The second type of rubber oxygenase has been named latex clearing protein (Lcp). Controversial reports were published on the cofactor of Lcp from Streptomyces sp. K30 (LcpK30) and G. polyisoprenivorans VH2 (LcpVH2)23, 24 but recently iron was detected in an almost 1:1 stoichiometry in pure preparations of LcpK30 and of LcpRr, and both Lcps were identified as b-type cytochromes. The typical, α-helical tertiary structure identifies LcpK30 as a member of the globin family. However, LcpK30 contains additional subdomains at the N- and C-termini beyond the globin core that form two caps located on opposite sides of the protein.

Here we report the three-dimensional structure of LcpK30 in a closed and in an open confirmation. His198 (F13) acts as the proximal axial ligand in LcpK30 and corresponds to His (F8) of GCSGsu according to the haemoglobin nomenclature. Interestingly, distal haem ligation in LcpK30 is not provided by a histidine as in most other globins and many cytochromes, but by a lysine residue (Lys167, E7) that corresponds to (His) E11 in GCSGsu and (His) E7 in haemoglobin. The presence of two axial ligands (His198, Lys167) to the haem iron in LcpK30 prevents the direct binding of dioxygen that is required for the dioxygenase activity of the enzyme and identifies this structure as a closed and inactive form. As a consequence, a conformational change in the vicinity of the haem group is required to allow for access and binding of O2 and of the polyisoprene chain to the haem site. The transition to the closed state only bars one entrance to this tunnel, but concomitantly blocks access to the haem iron by reinstating Lys167 as a direct ligand to the metal, thus efficiently preventing the reaction of the enzyme with dioxygen. Although LcpK30 is an extracellular enzyme, this conformational switch may well represent a protective mechanism to avoid the generation of reactive oxygen species from the reduced haem cofactor in the absence of substrate molecules. In summary, the findings for LcpK30 muteins with single amino acid exchanges of residues in the active site region were in agreement with the 5-fold-coordinated (open) state of the Lys167Ala mutein and with the 6-fold coordinated (closed) state in the wild type and in the Lys167His mutein with His167 as a second axial haem ligand. These data confirm that the unusual Lys167 haem ligand stabilises the protein in the absence of substrate in the closed state. z = 3.06 is typical for a low spin haem (Fe3+, S = 1/2), presumably from the closed state of the enzyme with Lys167 completing the octahedral coordination of the metal ion.

>[2x]PLWTWSPSASVAGTGVGVDPEYVWDEEADPVLAAVIDRGEVPAVNALLKQWTRNDQALPGGLPGDLREFMEHARRMPSWADKAALDRGAQFSKTKGIYVGALYGLGSGLMSTAIPRESRAVYYSKGGADMKDRIAKTARLGYDIGDLDAYLPHGSMIVTAVKTRMVHAAVRHLLPQSPAWSQTSGGQKIPISQADIMVTWHSLATFVMRKMKQWGVRVNTADAEAYLHVWQVSAHMLGVSDEYIPATWDAANAQSKQVLDPILAHTPEGEALTEVLLGIVAELDAGLTRPLIGAFSRYTLGGEVGDMIGLAKQPVLERLIATAWPLLVAFREGLIPLPAVPAVLWTLEEALRKFVLLFLSEGRRIAIDIPD16-hydroxyhexadecanoic acid | C16 H32 O3 | 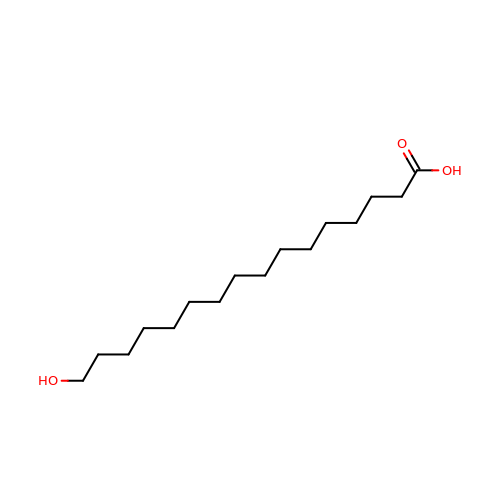UGAGPNKCDRTDHP-UHFFFAOYSA-N>[2x]MGSSHHHHHHSSGLVPRGSKNRPPFPWFGMDIGGTLVKLVYFEPKDITAEEEQEEVENLKSIRKYL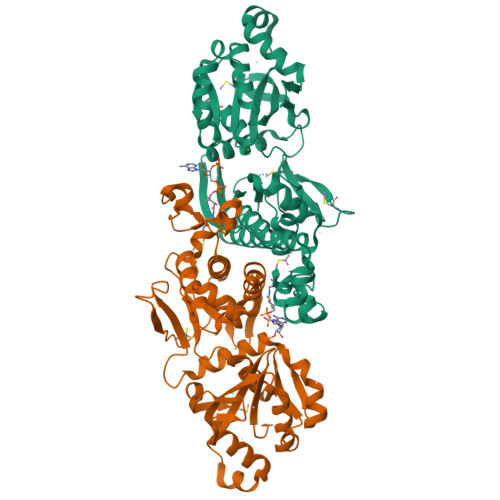TSNTAYGKTGIRDVHLELKNLTMCGRKGNLHFIRFPSCAMHRFIQMGSEKNFSSLHTTLCATGGGAFKFEEDFRMIADLQLHKLDELDCLIQGLLYVDSVGFNGKPECYYFENPTNPELCQKKPYCLDNPYPMLLVNMGSGVSILAVYSKDNYKRVTGTSLGGGTFLGLCCLLTGCETFEEALEMAAKGDSTNVDKLVKDIYGGDYERFGLQGSAVASSFGNMMSKEKRDSISKEDLARATLVTITNNIGSIARMCALNENIDRVVFVGNFLRINMVSMKLLAYAMDFWSKGQLKALFLEHEGYFGAVGALLELFKMTDD> MHKITPF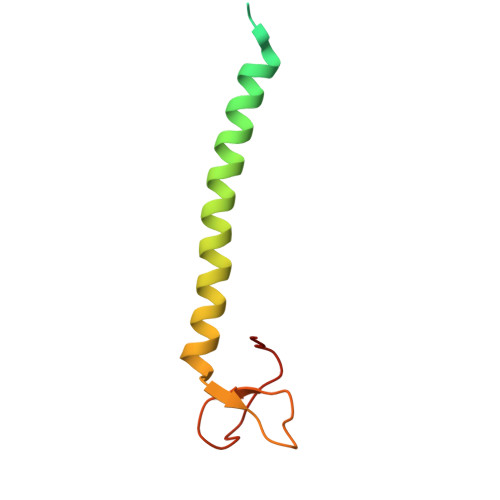LIAAVVAVIVLAVWLFKKDNKKETWFSRDLNYGKANSKIWNATVAKGLKGIANENAEIRKMYPYLGYGDFTGAICKGPNNQGCTYYANYTR>[14x]MLVFIDDGSTNIKLQWQESDGTIKQHISPNSFKREWAVSF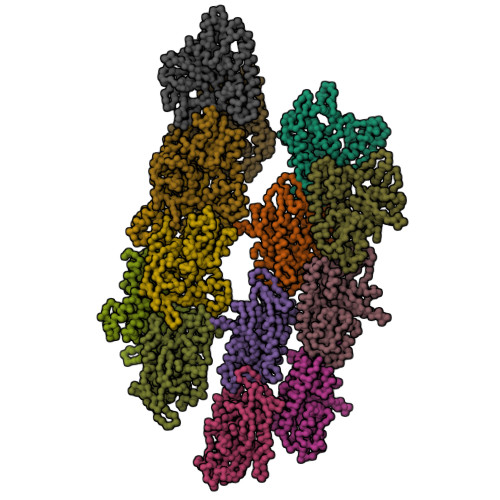GDKKVFNYTLNGEQYSFDPISPDAVVTTNIAWQYSDVNVVAVHHALLTSGLPVSEVDIVCTLPLTEYYDRNNQPNTENIERKKANFRKKITLNGGDTFTIKDVKVMPESIPAGYEVLQELDELDSLLIIDLGGTTLDISQVMGKLSGISKIYGDSSLGVSLVTSAVKDALSLARTKGSSYLADDIIIHRKDNNYLKQRINDENKISIVTEAMNEALRKLEQRVLNTLNEFSGYTHVMVIGGGAELICDAVKKHTQIRDERFFKTNNSQYDLVNGMYLI> MSIDSALNWDGEMTVTRFDSMTGAHFVIRLDSTQLGPAAGGTRAAQYSNLADALTDAGKLAGAMTLKMAVSNLPMGGGKSVIALPAPRHSIDPSTWARILRIHAENIDKLSGNYWTGPDVNTNSADMDTLNDTTEFVFGRSLERGGAGSSAFTTAVGVFEAMKATVAHRGLGSLDGLTVLVQGLGAVGGSLASLAAEAGAQLLVADTDTERVAHAVALGHTAVALEDVLSTPCDVFAPCAMGGVITTEVARTLDCSVVAGAANNVIADEAASDILHARGILYAPDFVANAGGAIHLVGREVLGWSESVVHERAVAIGDTLNQVFEISDNDGVTPDEAARTLAGRRAREASTTTATA;> MSIDSALNWDGEMTVTRFDKMTGAHFVIRLDSTQLGPAAGGTRAAQYSQLADALTDAGKLAGAMTLKMAVSNLPMGGGKSVIALPAPRHSIDPSTWARILRIHAENIDKLSGNYWTGPDVNTNSADMDTLNDTTEFVFGRSLERGGAGSSAFTTAVGVFEAMKATVAHRGLGSLDGLTVLVQGLGAVGGSLASLAA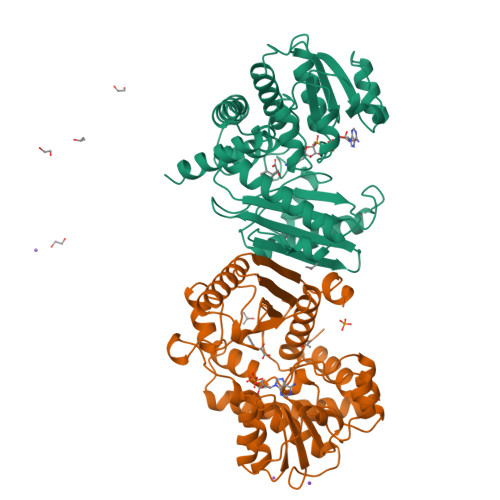EAGAQLLVADTDTERVAHAVALGHTAVALEDVLSTPCDVFAPCAMGGVITTEVARTLDCSVVAGAANNVIADEAASDILHARGILYAPDFVANAGGAIHLVGREVLGWSESVVHERAVAIGDTLNQVFEISDNDGVTPDEAARTLAGRRAREASTTTATA> GFKVFGAPNVVEDEIDQYLSKQDGKIYRSRDPQLCRHGPLGKCVHCVPLEPFDEDYLNHLEPPVKHMSFHAYIRKLTGGADKGKFVALENISCKIKSGCEGHLPWPNGICTKCQPSAITLNRQKYRHVDNIMFENHTVADRFLDFWRKTGNQHFGYLYGRYTEHKDIPLGIRAEVAAIYEPPQIGTQNSLELLEDPKAEVVDEIAAKLGLRKVGWIFTDLVSEDTRKGTVRYSRNKDTYFLSSEECITAGDFQNKHPNMCRLSPDGHFGSKFVTAVATGGPDNQVHFEGYQVSNQCMALVRDECLLPCKDAPELGYAKESSSEQYVPDVFYKDVDKFGNEITQLARP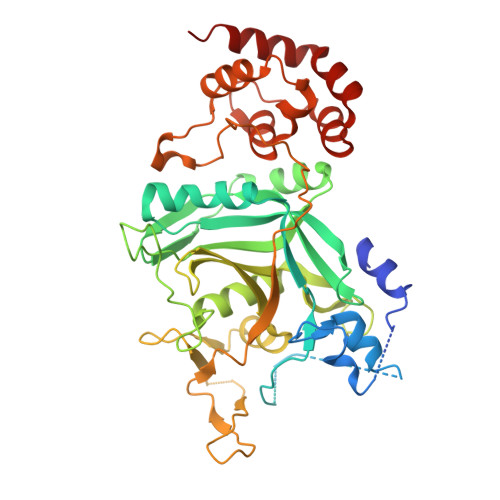LPVEYLIIDITTTFPKDPVYTFSISQNPFPIENRDVLGETQDFHSLATYLSQNTSSVFLDTISDFHLLLFLVTNEVMPLQDSISLLLEAVRTRNEELAQTWKRSEQWATIEQLCSTVG>MAKEVIVYTSNTCPHSFTVKEFLSENNVEFTEKNIQTDAAARKELMKKGIMAVPVIQIDEEVVVGFDRDKIEELLGLEH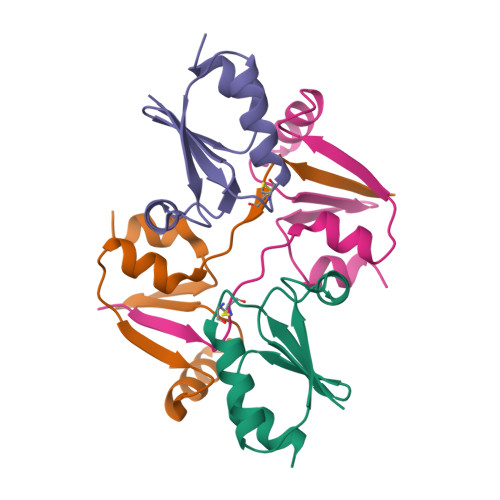HHHHH[4x]TRPV3 is most abundantly expressed in epidermal and hair follicle keratinocytes where it plays a key role in the maintenance of normal skin physiology. In contrast to other thermoTRP channels, TRPV3 sensitizes, rather than desensitizes, upon repeated stimulation with either heat or agonists. The TRPV3 channel, like other thermoTRPV channels (TRPV1, TRPV2, and TRPV427–30), is a fourfold symmetric homotetramer. Each monomer contains an amino- (N-) terminal cytosolic ankyrin repeat domain (ARD) and a domain-swapped transmembrane domain (TMD) comprising six transmembrane helices (S1−S6).

We determined the structure of full-length, human TRPV3T96A, hereafter simply referred to as TRPV3, in the closed apo state to ~3.4 Å using cryo-electron microscopy (cryo-EM). Extensive screening of various TRPV3 homologs and mutants identified human TRPV3 containing the point mutation T96A as optimal for structural studies. Characterization of both T96A and wild-type channels confirmed that the T96A mutation did not significantly alter the ligand-dependent gating profile of the TRPV3 channel. Third, we previously proposed that the presence of π-helices in the strategically important S4−S5 linker and S6 in TRPV channels likely acts as transient flexible hinge points that facilitate channel gating. Indeed, apo TRPV3 possesses a π-helix in the S4−S5 linker, whereas S6 is fully α-helical. In the apo structure, where the S6 helix is entirely α-helical, two pairs of interactions are present between S6 and the S4−S5 linker: one between residue N671 in S6 and the backbone carbonyl of Y575 located in the S4−S5 linker, and the other between the hydroxyl group of Y575 and the backbone amide of M672 within S6. Together, these interactions between S6 and the S4−S5 linker stabilize a straight, α-helical conformation of S6. Second, the selectivity filter (SF, residues 636–640) of TRPV3 is lined with backbone carbonyls, whereas the SFs of TRPV1 and TRPV2 are occluded by hydrophobic amino acid side-chains, such as methionine. Similarly to the SF in TRPV4, the TRPV3 SF is sufficiently wide (~7 Å) to permeate a semi-hydrated calcium ion. First, the high quality of the TRPV3 EM density map has allowed us to build the most complete thermoTRPV CTD to date (residues 707–754), a region that was not well resolved in the cryo-EM structures of TRPV1, TRPV2, or TRPV426–30. Notably, a thorough reanalysis of the apo TRPV3 datasets yielded no evidence of structural species containing symmetries lower than C4.

>MEKAHPKEMVPLMGKRVAAPSGNPAILPEKRPAEITPTKKSAHFFLEIEGFEPNPTVAKTSPPVFSKPMDSNIRQCISGNCDDMDSPQSPQDDVTETPSNPNSPSAQLAKEEQRRKKRRLKKRIFAAVSEGCVEELVELLVELQELCRRRHDEDVPDFLMHKLTASDTGKTCLMKALLNINPNTKEIVRILLAFAEENDILGRFINAEYTEEAYEGQTALNIAIERRQGDIAALLIAAGADVNAHAKGAFFNPKYQHEGFYFGETPLALAACTNQPEIVQLLMEHEQTDITSRDSRGNNILHALVTVAEDFKTQNDFVKRMYDMILLRSGNWELETTRNNDGLTPLQLAAKMGKAEILKYILSREIKEKRLRSLSRKFTDWAYGPVSSSLYDLTNVDTTTDNSVLEITVYNTNIDNRHEMLTLEPLHTLLHMKWKKFAKHMFFLSFCFYFFYNITLTLVSYYRPREEEAIPHPLALTHKMGWLQLLGRMFVLIWAMCISVKEGIAIFLLRPSDLQSILSDAWFHFVFFIQAVLVILSVFLYLFAYKEYLACLVLAMALGWANMLYYTRGFQSMGMYSVMIQKVILHDVLKFLFVYIVFLLGFGVALASLIEKCPKDNKDCSSYGSFSDAVLELFKLTIGLGDLNIQQNSKYPILFLFLLITYVILTFVLLLNMLIALMGETVENVSKESERIWRLQRARTILEFEKMLPEWLRSRFRMGELCKVAEDDFRLCLRINEVKWTEWKTHVSFLNEDPGPVRRTDFNKIQDSSRNNSKTTLNAFEEVEEFPETSVVDAGLEVLFQGPAAAVDYKDDDDKAHHHHHHHHHH[4x]>[60x]MSENEIQDQQPSDSMDGQRGGGGGATGSVGGGKGSGVGISTGGWVGGSYFTDSYVITKNTRQFLVKIQNNHQYKTELISPSTSQGKSQRCVSTPWSYFNFNQYSSHFSPQDWQRLTNEYKRFRPKGMHVKIYNLQIKQILSNGADTTYNNDLTAGVHIFCDGEHAYPNATHPWDEDVMPELPYQTWYLFQYGYIPVIHELAEMEDSNAVEKAICLQIPFFMLENSDHE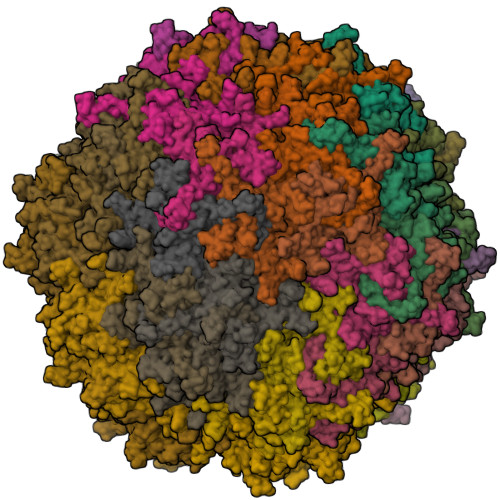VLRTGESTEFTFNFDCEWINNERAYIPPGLMFNPLVPTRRAQYIRRNNNPQTAESTSRIAPYAKPTSWMTGPGLLSAQRVGPATSDTGAWMVAVKPENASIDTGMSGIGSGFDPPQGSLAPTNLEYKIQWYQTPQGTNNNGNIISNQPLSMLRDQALFRGNQTTYNLCSDVWMFPNQIWDRYPITRENPIWCKKPRSDKHTTIDPFDGSLAMDHPPGTIFIKMAKIPVPSNNNADSYLNIYCTGQVSCEIVWEVERYATKNWRPERRHTTFGLGIGGADNLNPTYHVDKNGTYIQPTTWDMCFPVKTNINKVL>SNAMADGIYGSFENLKKHAGTMTLEAYMRFSAKLSEAKDEMGTKEYEVFTKELKKLTNAKLAYGDANGNIDYDALSPEKREEMKTVSMGLQPYFDKLNGHKSSKEVLTQEEFDRYMEALMTHEIVRVKTKSTGAIKVEEVPEAYKERFMKAEQFMEYVDEKVR[2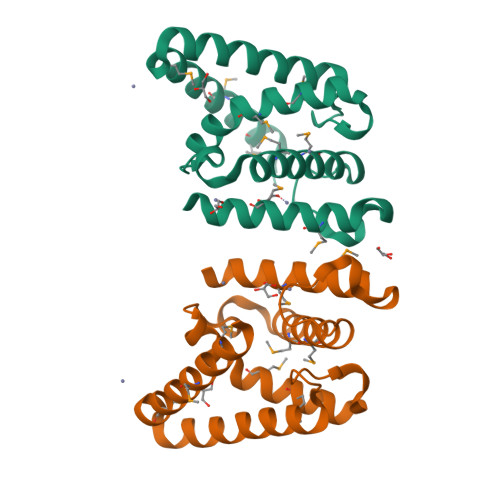x]> SATSAHSFTGRPLHIPPLPCPFPSEINEHADAVDEESHTWLAASHMLKGAD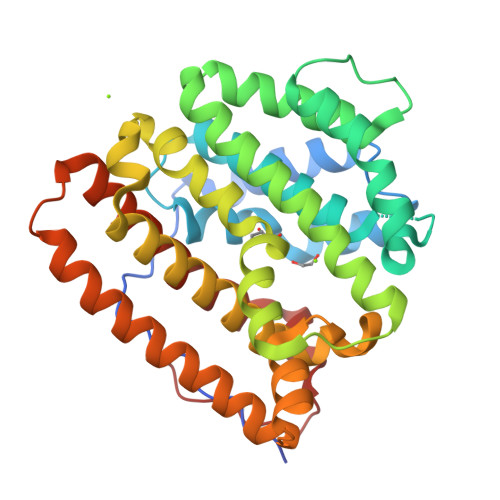TVEHFRRSKIGTLAARTNPTVPRDSLRLINDWYNWLFAFDDAFCEGELMGHRASALARALPPLLEILDGRREPDGSDAFGLALKELLHRISDVASPAQVDRWRTTVKEYLFAQIWEAANREVDLIPTPDDYVLMRRITGATYTCFALIDVGGGYRLEAEEWHHPDVRTLSDLACDLIGWDNDLLSYAKERGNDKARHNLVTVLATHKSLTLQDALLEVAQMHNDAVAAFLDRRAALDRWATLPVRKYVRGLEHWVRGHIAFSLGSARYVGAWPDDTRWPRAV> MHHHHHHSSGRENLYFQGETSVPPGSALVGPSCVMDDFRDPQRWKECAKQGKMPCYFDLIEENVYLTERKKNKSHRDIKRMQCECTPLSKDERAQGEIACGEDCLNRLLMIECSSRCPNGDYCSNRRFQRKQHADVEVILTEKKGWGLRAAKDLPSNTFVLEYCGEVLDHKEFKARVKEYARNKNIHYYFMALKNDEIIDATQKGNCSRFM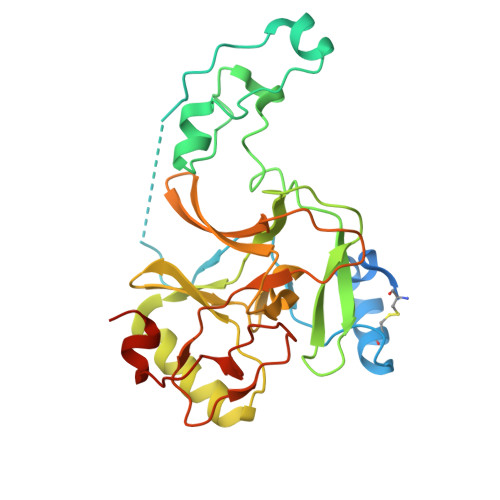NHSCEPNCETQKWTVNGQLRVGFFTTKLVPSGSELTFDYQFQRYGKEAQKCFCGSANCRGYLGGENRVSIRAAGGKMKKERSRK>[2x]MVRPSQSMYDRHLTIFSPDGNLYQIEYAIKAVKNTNITSVGVKGENCAVIISQKKMATQYISQDKLLDYNNITNIYNITDEIGCSMVGMPGDCLSMVYKARSEASEFLYSNGYNVNAETLCRNICDKIQVYTQHAYMRLHACSGMIIGIDENNKPELFKFDPSGFCAGYRACVIGNKEQESISVLERLLEKRKKKIQQETIDEDIRNTTILAIEALQTILAFDLKASEIEVAIVSTKNRNFTQISEKEIDNYLTYIAERD;>MADGEYSFSLTTFSPTGKLVQIEYALNRVSSSSPALGIRAKNGVIIATEKKSPNELIEENSIFKIQQISEHIGIVYAGMPGDFRVLLKRARKEAIRYSLQYGSEILVKELVKIIASIVQEFTQTGGVRPFGLSLLICGVDVYGYHLYQIDPSGCYFNWMATCVGKDYQNNMSFLEKRYNKDIEIEDAIHTAILTLKESYEGVLNEKNIEIGVAYDNKPFKILTQNEIKDYLIEIE[2x];>MARRYDSRTTTFSPEGRLYQVEYALEAINNASITIGLITKDGVILGADKVFISKLIDKANNYEKIYKIDKHIFCGVAGLNADANILINQSRLYAQRYLYNYNEVQPVSQLVVQICDIKQSYTQYGGLRPYGVSFLIGGYDTKDGYQLYHTDPSGNYSGWFATAIGTNNLTASSVLKQEWKNDMTLEEGLLLALKTLAKSTDTEIPKSEKIELAYLTNKDGEVYQKYLTEKEIEELIKLYTQKYIKE[2x];>[2x]MSYDRAITVFSPDGHLLQVEHALEAVKKGGCAVAIKSSNFAVLAVEKKNIPKLQNPKTTEKLIKLDEHNCLAFAGLNADARVLVNKTRLECQRYYLNMDEPAPVDYIAKYVAKVQQKFTHRGGVRPFGIATLIAGFKNNKEICIYQTEPSGIYAAWKAQAIGKNAKIVQEFLEKNYQENMEQKDCIFLALKAIFEVVELSSKNVEVALLTEKDLTFIEEQEINSMVELIDQERTKNNEQNE;>MFSTRSEYDRGVNTFSPEGRLFQVEYALGAIKLGSTAVGICVNDGVILASERRISSTLIEKDSVEKLLSIDDHIGCAMSGLMADARTLIDYARVECNHYKFIYNENINIKSCVELISELALDFSNLSDSKRKKIMSRPFGVALLIGGVDKNGPCLWYTEPSGTNTRFSAASIGSAQEGAELLLQENYKKDMTFEQAEILALTVLRQVMEDKLSTSNVEICAIKKSDQTFYKYNTDDISRIIDVLPSPVYPTIDMTA[2x];>[2x]MYRNLYDTDNIIYSPEGRLYQVEYASEAIKQGTCAVAIKSKDYVVVSGLKKCISKLSFPQEKIFKIDDYIGISMSGITSDAKVLTKFMQNECLSHKFLYNENINIESLVRSVADKYQKNTQKSSKRAFGVGLMIAAYHNEPCIFETRPNGSYFEYDALSFGARSHASKTYLEKNLHLFEECSLEELILHCLKALKCSLSSESELTISNTALAVVGKNHPWQEISSLQLEEYLSKVKMDAEQEQVEENVQNEANE;>MAGLSAGYDLSVSTFSPDGRLYQVEYIYKSINNNNTALCLECKDGIICCCINSNMDKNKMIKKNSYNRIYHVNNNIIITYSGFDGDARNIIDRARSEANTYYYNFHTNIPLHILVNRISLYIHAYTLYWHMRPFAASIIISSFNEKDKGDIYCIEPNGACYKYSGIVIGKNKEMFKTEIEKKDYKDINVRDAIEDIYKFILTSDDHM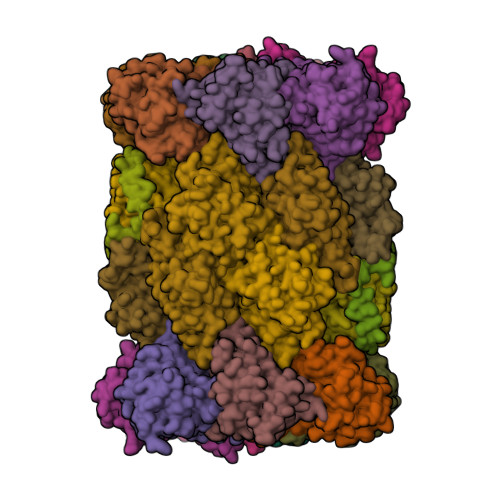NKNNLQNLVNFSWICKESSYEFQNIHEEILTPALNKAVEYIEKLN[2x];>[2x]TTIIGIIYDNGVMLACDSRTSSGTFISNKCSRKINRINENLYVCRSGASAHSQKIIEIIKHYCVSMKNENRKKGRFHEGETIYDETTYDEEIDIDSINYLDYNNNNDNNLVTKNKYFYEDKFNDYNPLVENVAHITKKIIYTNNNFLSCALIFGGYDKIKKQQLYAVNLNGSIIEKHDFAVSGSGSIYIQSYLQDKYKKFMTKKECFNLILNCVKYAMHNDNSSGGLIRIVNITKSFVEEFTVVNTQMNFQY;>[2x]TTICGLVCQNAVILGADTRATEGPIVADKNCSKLHYISKNIWCAGAGVAGDLEHTTLWLQHNVELHRLNTNTQPRVSMCVSRLTQELFKYQGYKVCAIVLGGVDVNGPQLYGIHPHGSSCLLPFTALGSGSLNAMAVLEAKYRDNMTIEEGKNLVCEAICAGIFNDLGSGGNVDICVITKDSYQHIRPYKEPNMRLYHLPHPTIYPKGTTPILSEKIEYIKKFISVEDA;>[2x]MGSIYNYNGGCVLGMSGSNCVAIACDLRLGANTFTTVSTKFSKIFKMNNNVYVGLSGLATDIQTLYEILRYRVNLYEVRQDAEMDVECFANMLSSILYSNRFSPYFVNPIVVGFKLKHYVDEEGEKKVNYEPYLTAYDLIGAKCETRDFVVNGVTSEQLFGMCESLYVKDQDENGLFETISQCLLSALDRDCISGWGAEVLVLTPEKIIKKKLKARMD;>[2x]MDTLIGLRGNNFVVLAADTYSINSIIKLKNDDNTKFYDIHGNKCLLLGGSIGDRLQFGEFIRKNVHLYQYQNNTDMFVKSFAFFTRKNLAYYLRRNPFEVNCLIAGYDKKDGYQLYWCDYLSNMDSVNKGAHGYGAYLVSAILDKYYHENLTVDEALDIFKLCFEELKKRFLLTQINYELRIMYDNKVETQYVTV;>TTTLAFKFKDGIIVAVDSRASMGSFISSQNVEKIIEINKNILGTMAGGAADCLYWEKYLGKIIKIYELRNNEKISVRAASTILSNILYQYKGYGLCCGIILSGYDHTGFNMFYVDDSGKKVEGNLFSCGSGSTYAYSILDSAYDYNLNLDQAVELARNAIYHATFRDGGSGGKVRVFHIHKNGYDKIIEGEDVFDLHYHYTNPEQKDQYVM[2x];>MDLILYNDNLTEKKTEKENVIEHGRGFKRWYPYIDNGGTVIGLTGKDYVILAADTRLSLSYSIYTRFCPKISKLTDKCIIGSSGMQSDIKTLHSLLQKKIQLFVLEHSHYPDIHVIARLLCVILYSRRFFPYYAFNILAGVDENNKGVLYNYDSVGSYCEATHSCVGSGSQLILPILDNRVEQKNQLIKNTNFNLGDDINFVKDAITSATERDIYTGDKTLIYVIDKMGINVNTLDLKQD[2x];>MTLGPVVTGTSVIAIKYKHGIMIAADRKASYGSYAKFQNVERIFKINNKTVMGFSGELADAQYLHELLTRKNINNLSEKKRKEDMYTPQHYHSYVSRVFYVRKNRIDPLFNNIIIAGINSQKYDNNDDNVLLYTNKNNDDEQNEYKNNEEYKEIHKDDLYIGFVDMHGTNFCDDYITTGYARYFALTLLRDHYKDNMTEEEARILINECLRILYFRDATSSNFIQIVKVTSKGVEYEEPYILPCVLNSADYVYPSTLLPPAGCMW[2x]> NQRF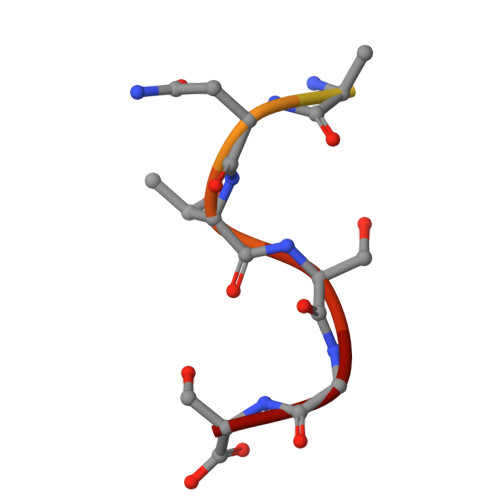GSNNTSGS4-({[(3R,4R)-4-{[3-methyl-5-(5-methylpyridin-3-yl)-2-oxo-1,2-dihydro-1,7-naphthyridin-8-yl]amino}piperidin-3-yl]oxy}methyl)-1lambda~6~-thiane-1,1-dione 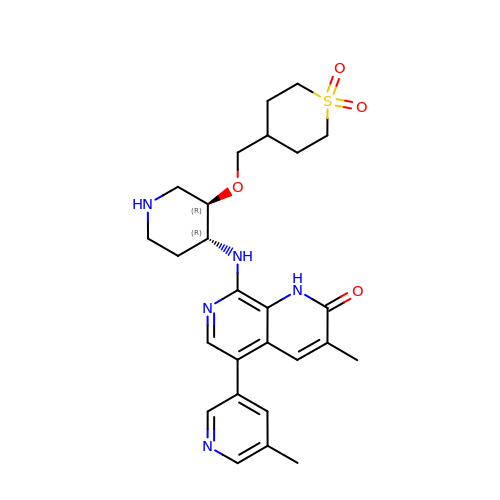| C26 H33 N5 O4 S | ZIRMKCLZUOCUSC-DHIUTWEWSA-N>[2x]HQYLLPEAKAQDSDKICVVINLDETLVHSSFKPVNNADFIIPVEIDGVVHQVYVLKRPHVDEFLQRMGELFECVLFTASLAKYADPVADLLDKWGAFRARLFRESCVFHRGNYVKDLS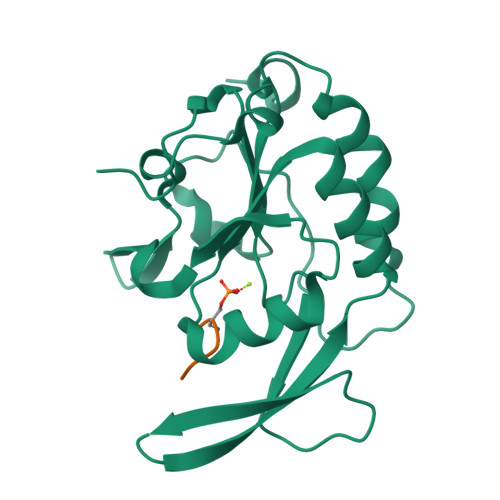RLGRDLRRVLILDNSPASYVFHPDNAVPVASWFDNMSDTELHDLLPFFEQLSRVDDVYSVLRQ;>SYSPTSPS[2x]> GSHMAYTLKVHYKYTVVMKTQPGLPYSQVRDMVSKKL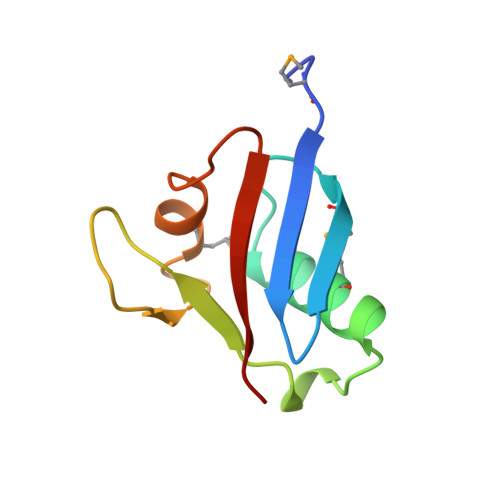ELRLEHTKLSYRPRDSNELVPLSEDSMKDAWGQVKNYCLTLWCENT>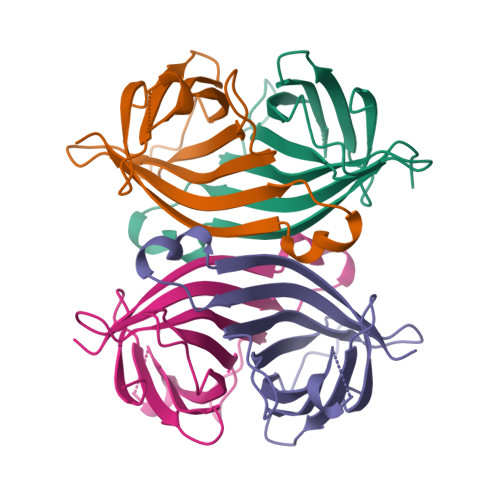AEAGITGTWYNQLGSTFIVTAGADGALTGTYESAVGNAESRYVLTGRYDSAPATDGSGTALGWTVAFKNNYRNAHSATTWSGQYVGGAEARINTQWLLTSGTTEANAWKSTLVGHDTFTKVKPSAAS[4x]>[2x]MPAPVLSGPQYLREGLKLVLSPGLRLFVLLPLLINLVLFVGLIYFAGHQFSLWVDALMPSLPHWLSFLNYLLWPLFVVLVALMVFFTFTMLANIIAAPFNGFLSEKVEAVVRGVDNSPPFSWGELIAMVPRTLAREMRKLGYFLPRAIALLILS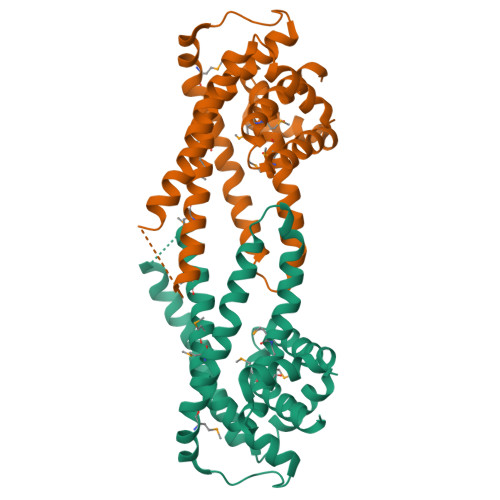FIPVLNLVAAPLWLIFGVWMMAIQYIDYPADNHKLGWNEMLAWLREKRWQSLSFGGIVYLVLLIPVVNILMMPAAVAGATLFWVRERGDEALARTRA> MSNSIEAKLQEDLRDALVDYYLGQIVPNSKDFTNLRSTIKNVDDLYDHLLLDTQVSAKVITSRLSLVTQSVQQYINRIALNLEPGLSINQQEATDWEEFANRYGYWAANQQLRMFPEIYVDPTLRLTKTEFFFQLESALNQGKLTDDVAQKAVLGYLNNFEEVSNLEIIAGYQDGIDIENDKTYFVARTRMQPYRYFWRSLDASQRNANSQELYPTAWSEWKAISVPLENVANGIVRPIMMDNRLYISWFEVAEEKETDSDGNIIVSGRYRTKIRLAHLGFDGVWSSGTTLREEVLADQMEEMIAVVDRMEDEPRLALVAFKEMSESWDVVFSYICDSMLIESSNLPTTTHPPKPGDGDKGLSDLDDYGANLVWFYLHETANGGKAEYKQLILYPVIINRDWPIELDKTHQGDFGTVDDFTLNSNYTGDELSLYLQSSSTYKYDFSKSKNIIYGIWKEDANNNRCWLNYKLLTPEDYEPQINATLVMCDKGDVNIITGFSLPNGGVDAGGKIKVTLRVGKKLRDKFQIKQFSQTQYLQFPEASSADVWYIGKQIRLNTLFAKELIGKASRSLDLVLSWETQNSRLEEAILGGAAELIDLDGANGIYFWELFFHMPFMVSWRFNVEQRYEDANRWVKYLFNPFECEDEPALLLGKPPYWNSRPLVDEPFKGYSLTQPSDPDAIAASDPIHYRKAVFNFLTKNIIDQGDMEYRKLQPSARTLARLSYSTASSLLGRRPDVQLTSFWQPLTLEDASYKTDSEIRAIEMQSQPLTFEPVVHDQTMSAVDNDIFMYPMNNELRGLWDRIENRIYNLRHNLTLDGKEINMDLYDSSISPRGLMKQRYQRVVTARNASKMNFKVPNYRFEPMLNRSKSGVETLIQFGSTLLSLLERKDSLSFDAYQMIQSGDLYRFSIDLQQQDIDINKASLEALQVSKQSAQDRYDHFKELYDENISSTEQKVIELQSQAANSLLMAQGMRTAAAALDVIPNIYGLAVGGSHWGAPLNAAAEIIMIKYQADSSKSESLSVSESYRRRRQEWEL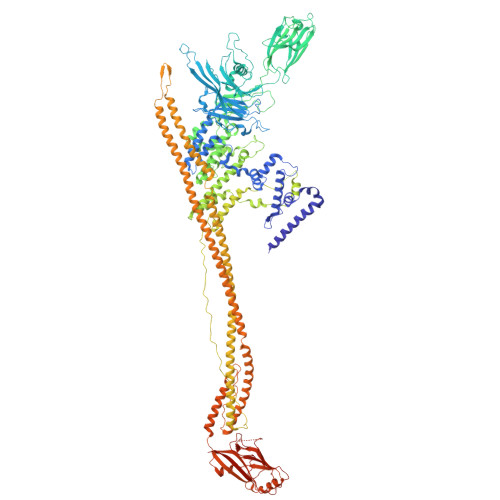QYKQAEWEVNSVEQQINLQNMQIKAANKRLEQVEAQQQQAMALLDYFSERFTNESLYTWLISQLSSLYLQAYDAVLSLCLSAEASLLYELNLGEQSFVGGGGWNDLYQGLMAGETLKLALMRMERVYVEQNSRRQEITKTISLKALLGESWPAELNKLKQKTPINFNLEEQIFVEDYQELYQRRIKSVSVSLPMLVGPYEDVCAQLTQTSSSYSTRADLKTVENMLTKRTFADTPHLVRSIQPNQQISLSTGVNDSGLFMLNFDDERFLPFEGSGVDSSWRLQFTNLKQNLDSLNDVILHVKYTAAIGSSTFSQGVRKILANINNDE> MSEKTTKGVQLLRGDPKKAIVRLSIAMMIGMSVQTLYNLADGIWVSGLG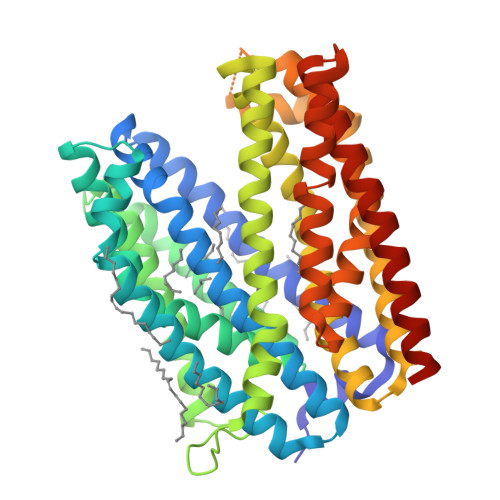PESLAAVGLFFPVFMGIIALAAGLGVGTSSAIARRIGARDKEGADNVAVHSLILSLILGVTITITMLPAIDSLFRSMGAKGEAVELAIEYARVLLAGAFIIVFNNVGNGILRGEGDANRAMLAMVLGSGLNIVLDPIFIYTLGFGVVGAAYATLLSMVVTSLFIAYWLFVKRDTYVDITLRDFSPSREILKDILRVGLPSSLSQLSMSIAMFFLNSVAITAGGENGVAVFTSAWRITMLGIVPILGMAAATTSVTGAAYGERNVEKLETAYLYAIKIAFMIELAVVAFIMLFAPQVAYLFTYSESAQVIKGDLISALRTLPVFLVLTPFGMMTSAMFQGIGEGEKSLILTIFRTLVMQVGFAYIFVHYTTLGLRGVWIGIVIGNMVAAIVGFLWGRMRISALKKTSATGGKR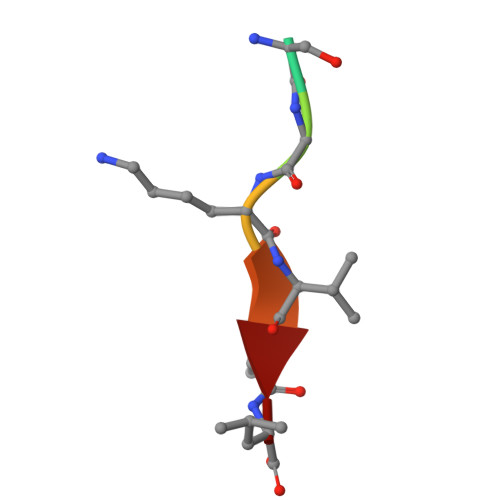> SSGKVPL[2-AMINO-3-(4-HYDROXY-PHENYL)-PROPIONYLAMINO]-(1,3,4,5-TETRAHYDROXY-4-HYDROXYMETHYL-PIPERIDIN-2-YL)- ACETIC ACID | C17 H25 N3 O9 | 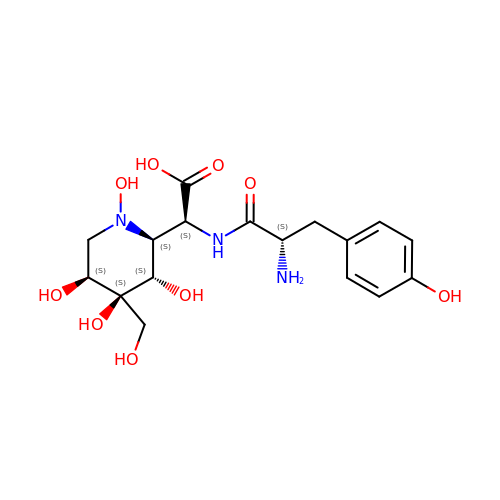YNVYTCBBBGXDHW-NCBDHNCWSA-N N-{[(1S)-5-{4-[25-({2,4-BIS[HYDROXY(OXO)AMMONIO]PHENYL}AMINO)-2,5,8,11,14,17,20,23-OCTAOXAPENTACOS-1-YL]-1H-1,2,3-TRIAZOL-1-YL}-1-CARBOXYPENTYL]CARBAMOYL}-L-GLUTAMIC ACID | 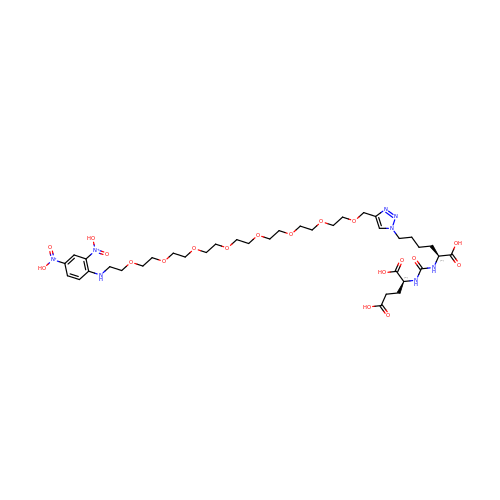C37 H60 N8 O19 | DIUDJPQWCLVKSG-ACHIHNKUSA-P>[6x]XGELAAIKQELAAIKKELAAIK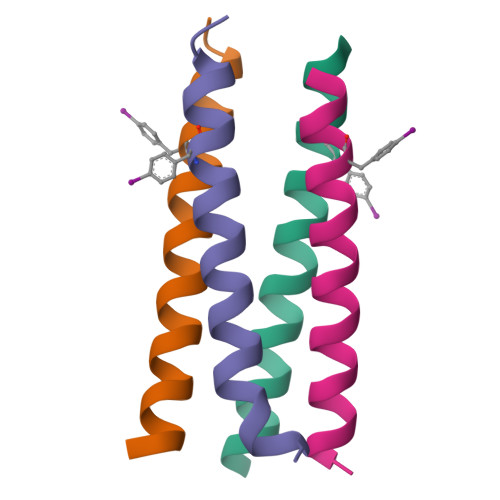FELAAIKQGAGX Phage portal proteins are key viral components located in a single pentameric vertex of the capsid and they act as initiators of capsid assembly. They are also critical components of the DNA-packaging complex and are involved in tail assembly. Here we report a number of crystal and high-resolution cryo-electron microscopy (cryo-EM) structures of the T7 bacteriophage portal (gp8). The structures show two conformations—open and closed—of the portal and suggest a possible mechanism of the channel valve that regulates DNA passage.

A second cryo-EM data set yielded a higher resolution map than the initial one used for phasing. This map at 4.1 Å resolution shows a different conformation of the 12mer portal (gp8open). The overall structure is similar to that already described (RMSD 1.03 Å), with the exception of the conformation of the channel α10 helix, which is kinked in the middle and deviates “upwards,” instead of pointing perpendicular toward the channel axis. The kink occurs at a region containing two adjacent glycine residues (G386 and G387), which provide the necessary flexibility to change the orientation of the N-terminal half of the helix. The movement represents a large swing of 90°. The density corresponding to the tunnel loop is partially visible and reveals that it is in an extended conformation, allowing the connection of the now more distant α9 and α10 helices. In gp8open, the kinked part of helix α10 occupies the “upper” cavity of the channel or α10 housing cavity, thus defining a larger conical channel instead of the two inverted conical cavities observed in gp8closed. Therefore, two clearly different conformations in the T7 connector were defined: one closed (gp8closed) and the other open (gp8open). Although the first structure described in this work (gp8closed) would impede the DNA passage through it, the second structure (gp8open) would allow it.

>MAEKRTGLAEDGAKSVYERLKNDRAPYETRAQNCAQYTIPSLFPKDSDNASTDYQTPWQAVGARGLNNLASKLMLALFPMQTWMRLTISEYEAKQLLSDPDGLAKVDEGLSMVERIIMNYIESNSYRVTLFEALKQLVVAGNVLLYLPEPEGSNYNPMKLYRLSSYVVQRDAFGNVLQMVTRDQIAFGALPEDIRKAVEGQGGEKKADETIDVYTHIYLDEDSGEYLRYEEVEGMEVQGSDGTYPKEACPYIPIRMVRLDGESYGRSYIEEYLGDLRSLENLQEAIVKMSMISSKVIGLVNPAGITQPRRLTKAQTGDFVTGRPEDISFLQLEKQADFTVAKAVSDAIEARLSFAFMLNSAVQRTGERVTAEEIRYVASELEDTLGGVYSILSQELQLPLVRVLLKQLQATQQIPELPKEAVEPTISTGLEAIGRGQDLDKLERCVTAWAALAPMRDDPDINLAMIKLRIANAIGIDTSGILLTEEQKQQKMAQQSMQMGMDNGAAALAQGMAAQATASPEAMAAAADSVGLQPGIAAALEHHHHHH[12x]> ISRLGPDSDFLTSVVAKASTSIVTPADRILVKQPLSASSF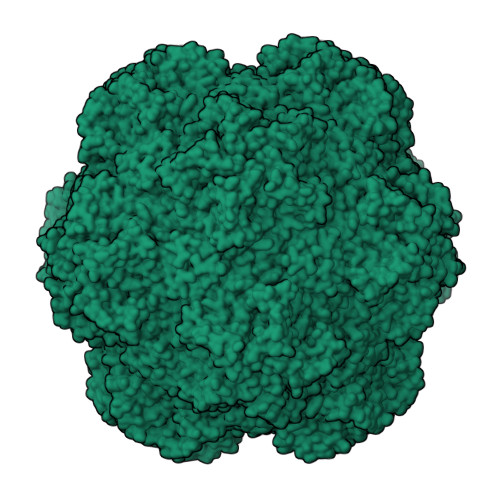PGTRITGLSSYWERYKWLSAVARYVPAVPNTVACQFVMYIDTDPLDDPSNISDDNQIVRQAVSQAGSNQFNFNTSKTVPLIVRADNQYYYTGVDKQNLRFSLQGILYIIQVTDLINFNGELITQDLTCGSLFLDWLVNFSIPQIN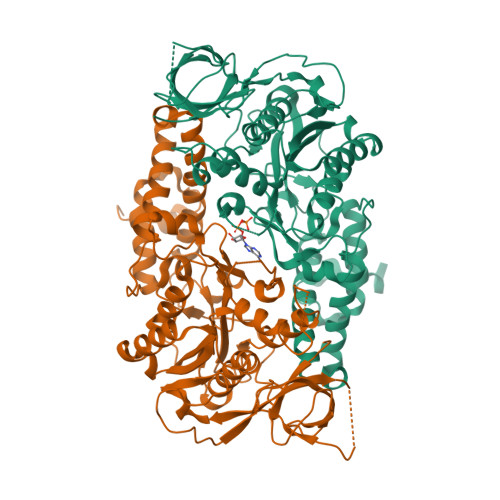>[2x]MKHHHHHHPMVKEYKTITQIAGPLIFVEKTEPVGYNEIVNIKMGDGTVRRGQVLDSSADIVVVQVFEGTGGLDKDCGVIFTGETLKLPASVDLLGRILSGSGEPRDGGPRIVPDQLLDINGAAMNPYARLPPKDFIQTGISTIDGTNTLVRGQKLPIFSASGLPHNEIALQIARQASVPGSESAFAVVFAAMGITNEEAQYFMSDFEKTGALERAVVFLNLADDPAVERIVTPRMALTAAEYLAYEHGMHVLVILTDITNYAEALRQMGAARNEVPGRRGYPGYMYTDLATLYERAGIVKGAKGSVTQIPILSMPGDDITHPIPDLSGYITEGQIVVARELHRKGIYPPINVLPSLSRLMNSGIGAGKTREDHKAVSDQMYAGYAEGRDLRGLVAIVGKEALSERDTKFLEFADLFEDKFVRQGRNENRTIEDTLEIGWQILTHLPENQLGRIDNKYIQKYHPAHRKAK> MSRSG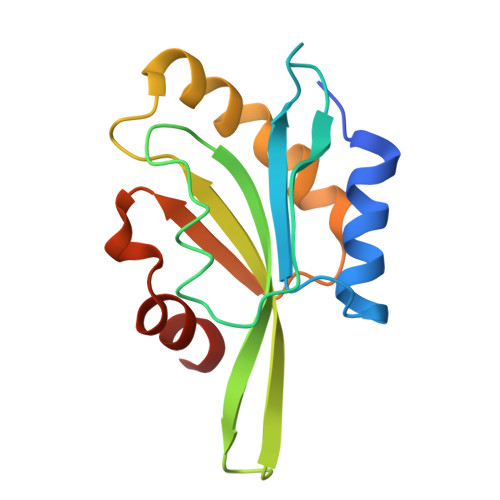VAVADESLTAFNDLKLGKKYKFILFGLNDAKTEIVVKETSTDPSYDAFLEKLPENDCLYAIYDFEYEINGNEGKRSKIVFFTWSPDTAPVRSKMVYASSKDALRRALNGVSTDVQGTDFSEVSYDSVLERVSRGAGSH>[2x]HHHHHHMLKVGFIGWRGMVGSVLMSRMIESKDFDCILPTFFSTSQVGQLPTGFMQQYGALQDAYSIDQLSSMDILLSCQGGEYTKEIHHKLREAGWQGFWIDAASTLRLDKDSTLVLDPL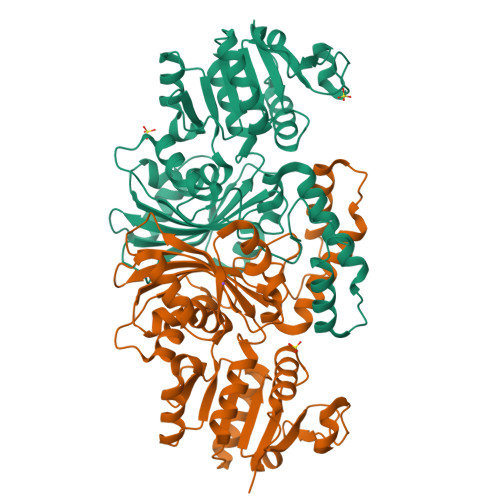NHDQIINAIDNGKKDFIGSNCTVSLMSLAIAGLLKEDLVEWVNSSTYQAISGAGAAAMQELLQQTSLLSKIDNRDEDILIREKILRELSKDSSKIPQQKTVQTLAYNLLPWIDVGMPSGQTKEEYKAATELNKILDTKKTIPVDGICVRVPSLRSHSQALTVKLRQKLTIEEIKQKISQGNEWVKVIDNNKEDTLKYLTPQANSGTLDIAIGRIKSSLLADDIFHCFTVGDQLLWGAAEPLRRVLNIIKI> TGGTHTPKLKHLDKLLAHCHRRRYTAKSTIIYAGDRCETLFFIIKGSVTILIEDDDGREMIIGYLNSGDFFGELGLFEKEGSEQERSAWVRAKVECEVAEISYAKFRELSQQDSEILYTLGSQMADRLRKTTRKVGDLAFLDVTGRVARTLLDLCQQPDAMTHPDGMQIKITRQEIGRIVGCSREMVGRVLKSLEEQGLVHVKGKTMVVFGTR;> TGGTHTPKLKHLDKLLAHCHRRRYTAKSTIIYAGDRCETLFFIIKGSVTILIEDDDGREMIIGYLNSGDFFGELGLFEKEGSEQERSAWVRAKVECEVAEISYAKFRELSQQDSEILYTLGSQMADRLRKTTRKVGDLAFLDVTGRVARTLLDLCQQPDAMTH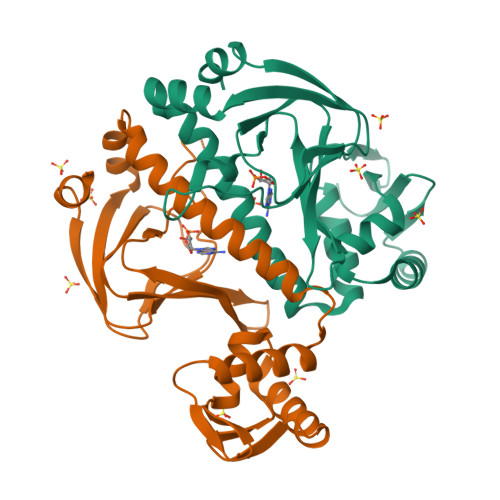PDGMQIKITRNEIGRIVGCSREMVGRVLKSLEEQGLVHVKGKTMVVFGTR Chlorogenic acid | C16 H18 O9 | 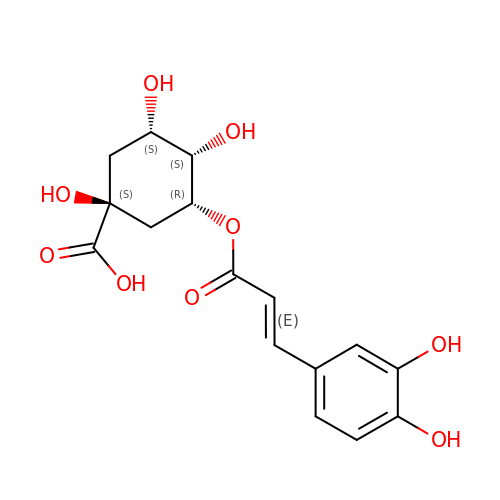CWVRJTMFETXNAD-FWCWNIRPSA-N> GPLGSPEFEPKLGQPVEWTPCRSSNPQVKIPGGALCGKLAVPVDYDRPDGDVAALALIRFPATGDKIGSLVINPGGPG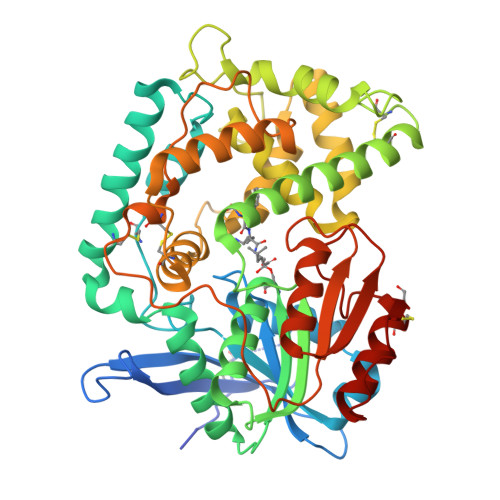ESGIEAALGVFQTLPKRVHERFDLVGFDPRGVASSRPAIWCNSDADNDRLRAEPQVDYSREGVAHIENETKQFVGRCVDKMGKNFLAHVGTVNVAKDLDAIRAALGDDKLTYLGYSYGTRIGSAYAEEFPQRVRAMILDGAVDPNADPIEAELRQAKGFQDAFNNYAADCAKNAGCPLGADPAKAVEVYHSLVDPLVDPDNPRISRPARTKDPRGLSYSDAIVGTIMALYSPNLWQHLTDGLSELVDNRGDTLLALADMYMRRDSHGRYNNSGDARVAINCVDQPPVTDRDKVIDEDRRAREIAPFMSYGKFTGDAPLGTCAFWPVPPTSQPHAVSAPGLVPTVVVSTTHDPATPYKAGVDLANQLRGSLLTFDGTQHTVVFQGDSCIDEYVTAYLIGGTTPPSGAKC>[3x]MVQTSFEHHHHHHSAGENLYFQGAQISMRLYSNRDRPNHLGPLALERLARVDDVVAQPARQPEDGFAASEDSLLGDVEEYARLFTRFLDGPVAPLGDAIPDDPARRAENLKASAYFLDASMVGICRLDPDDRAGDCDPSHTH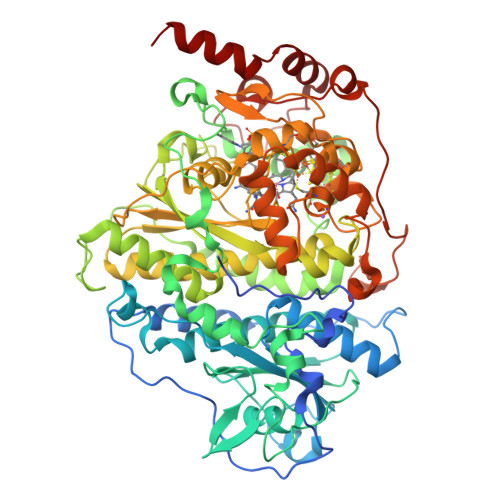ALVFAVQFGREPEAGEAGAEWIRGTNAARTDMRCAEIAAILSGYVRWMGFPARGHFSGDAQVDLARLAVRAGLARVVDGVLVAPFLRRGFRLGVVTTGYALAADRPLAPEGDLGETAPEVMLGIDGTRPGWEDAEEEKRPLHMGRYPMETIRRVDEPTTLVVRQEIQRVAKRGDFFKRAEAGDLGEKAKQEKKRFPMKHPLALGMQPLIQNMVPLQGTREKLAPTGKGGDLSDPGRNAEAIKALGYYLGADFVGICRAEPWMYYASDEVEGKPIEAYHDYAVVMLIDQGYETMEGASGDDWISASQSMRAYMRGAEIAGVMAAHCRRMGYSARSHSNAHSEVIHNPAILMAGLGEVSRIGDTLLNPFIGPRSQSIVFTTDLPMSVDRPIDFGLQDFCNQCRKCARECPCNAISFGDKVMFNGYEIWKADVEKCTKYRVTQMKGSACGRCMKMCPWNREDTVEGRRLAELSIKVPEARAAIIAMDDALQNGKRNLIKRWWFDLEVIDGVAGAPRMGTNERDLSPDRGDKIGANQKLAMYPPRLQPPPGTTLDAVLPVDRSGGLAEYAAAETPAAARARLKSSAG>MTLFPVLNNTPVGKQVDSIYESRLDQFLSEGQYRDFNLPSVYDHARIDNPSGDVNNDLSKGFVDLKVYRVPDLSRPSFNEVVGHKKFDETASKGDTFGPSWATFWFEVHIRLPKSWAKYEQVIFQWNCDNEGLVYSQDGVPLQAFSGSERTDFILPDSWKTTEDTFYIEMACNGMFGTGAGSQIAPPDPNRYFTLTKADLVAPNLPAMALAYDFLLMQQCVKQLPSNCWQKYKARQICNDIMNTFHPNDLSTINECRNLAKAFLGNDIDSEAVFEKNNDKANVFAIGHCHIDTAWLWPFAETRRKIVRSWATQMNIMDRYPEYQFVCSQALQYLWLKEDHPDVFEKLKEYVNQNKFIPIGGSWVEHDTNIPNGESLIRQFLLGQHFFEKEFGVRCRTFWLPDTFGYSSQIPQICRLCGMDRFLTQKLSWNNINSFPTSTFNWVALDGSQVICHMPPANTYTADTNVNDVLHSIDQHKNLVNDQAGLLVFGIGDGGGGPTPEMLEKLRRCKGIANTVGYLPNVKLGNTVDEFFDGILKRTNAGQTLPSWNGELYFEFHRGTYTTQAELKKLMRKVEIALHDAEYVSTLASIFSKDYSYPKESLQDLWRDTLLCQFHDVLPGSCIEMVYKDAIPIMSKVLKNTEALLWQAIEQLGFKKASSSDNKEQLCLLNTLPWNVRGVITETEENKLVYFESCDGKGILTAAHTSLKHPAAAYQKDDNFILVNDHLRVTIAPNGLILSLFDLHKEREILDLKSGKNHAGANQYVLFEDTPLSWQAWDTEVFSLEKYEVLDKGKVSIKESGPLRASVVVDIPISELSHMKATISLEGYNDCSEFTGVNFTCEVDWHESCKFLKVEFPVDIHSEFASYETQFGITKRPTHYNTSWDVAKFEVCHQKFADYSDFTYGVSVLNDCKYGFSTHGNLMRLSLLRSPKQPDAHADMGKHTIRYAVYPHSKPLDSSTVRAAHKFNSNFRLLTRASDTANLDIFDAFQLVGEPNVILSHIKMAEKGKSIILRVYESLGGKSRARLVIKSLTVASVTKCNGLEEDLEELCTLKSNDYYEVPIELRAFEIATFKVNLGSMSKGKVVDIMDYKDDDDKPMDYKDDDDKHHHHHHDELYKRSGAPLLNKRISYDL[4x]

Fungal α‐mannosidase Ams1 and its mammalian homolog MAN2C1 hydrolyze terminal α‐linked mannoses in free oligosaccharides released from misfolded glycoproteins or lipid‐linked oligosaccharide donors. Ams1 is transported by selective autophagy into vacuoles.

Here, we determine the tetrameric structure of Ams1 from the fission yeast Schizosaccharomyces pombe at 3.2 Å resolution by cryo‐electron microscopy. Distinct from a low resolution structure of S. cerevisiae Ams1, S. pombe Ams1 has a prominent N‐terminal tail that mediates tetramerization and an extra β‐sheet domain. Ams1 shares a conserved active site with other enzymes in glycoside hydrolase family 38, to which Ams1 belongs, but contains extra N‐terminal domains involved in tetramerization. The atomic structure of Ams1 reported here will aid understanding of its enzymatic activity and transport mechanism.> MVPGSEGPARAGSVVADVVFVIEGTANLGPYFEGLRKHYLLPAIEYFNGGPPAETDFGGDYGGTQYSLVVFNTVDCAPESYVQC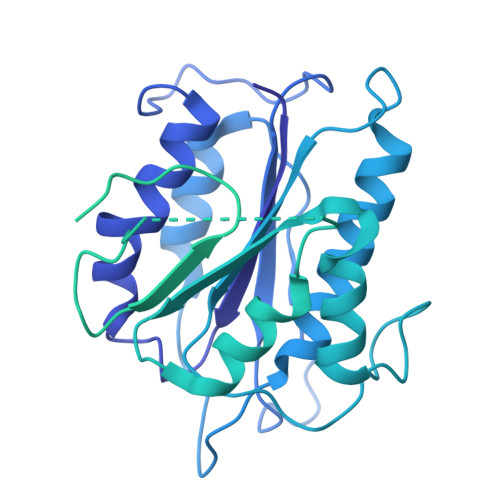HAPTSSAYEFVTWLDGIKFMGGGGESCSLIAEGLSTALQLFDDFKKMREQIGQTHRVCLLICNSPPYLLPAVESTTYSGCTTENLVQQIGERGIHFSIVSPRKLPALRLLFEKAAPPALLEPLQPPTDVSQDPRHMVLVRGLVLPVGGGSAPGPLQSKQPVPLPPAAPSGATLSAAPQQPLPPVPPQYQVPGNLSAAQVAAQNAVEAAKNQKAGLGPRFSPITPLQQAAPGVGPPFSQAPAPQLPPGPPGAPKPPPASQPSLVSTVAPGSGLAPTAQPGAPSMAGTVAPGGVSGPSPAQLGAPALGGQQSVSNKLLAWSGVLEWQEKPKPASVDANTKLTRSLPCQVYVNHGENLKTEQWPQKLIMQLIPQQLLTTLGPLFRNSRMVQFHFTNKDLESLKGLYRIMGNGFAGCVHFPHTAPCEVRVLMLLYSSKKKIFMGLIPYDQSGFVNGIRQVITNHKQVQQQKLEQQQRGMGGQQAPPGLGPILEDQARPSQNLLQLRPPQPQPQGTVGASGATGQPQPQGTAQPPPGAPQGPPGAASGPPPPGPILRPQNPGANPQLRSLLLNPPPPQTGVPPPQASLHHLQPPGAPALLPPPHQGLGQPQLGPPLLHPPPAQSWPAQLPPRAPLPGQMLLSGGPRGPVPQPGLQPSVMEDDILMDLI ethyl (1,1-dioxo-1lambda~6~,4-thiazinan-4-yl)acetate 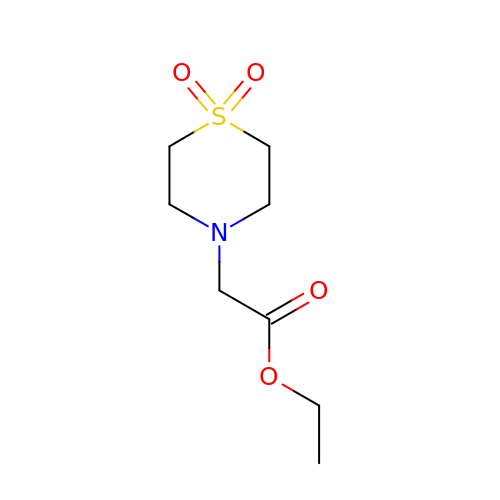| C8 H15 N O4 S | KWVBKMSCALADDC-UHFFFAOYSA-N(R)-1-PARA-NITRO-PHENYL-2-AZIDO-ETHANOL | C8 H8 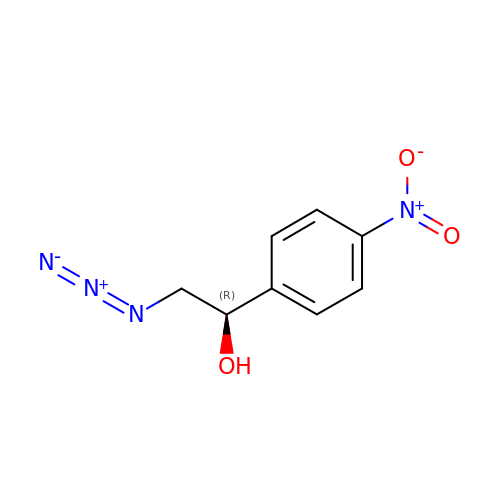N4 O3 | DHEGJYKMZJGYGW-QMMMGPOBSA-N> 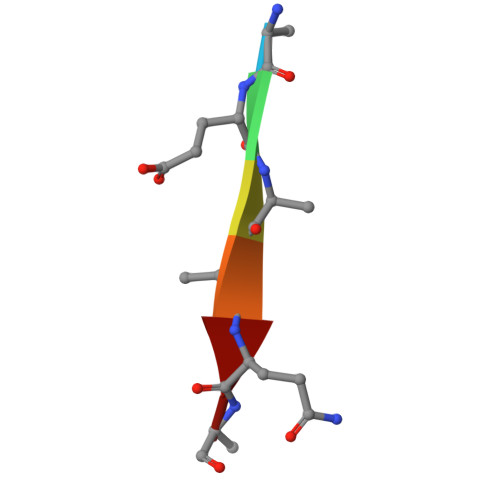AEAAQA3-(AMINOCARBONYL)-1-[(2R,3R,4S,5R)-5-({[(S)-{[(S)-{[(2R,3S,4R,5R)-5-(2-AMINO-6-OXO-1,6-DIHYDRO-9H-PURIN-9-YL)-3,4-DIHYDROXYTETRAHYDROFURAN-2-YL]METHOXY}(HYDROXY)PHOSPHORYL]OXY}(HYDROXY)PHOSPHORYL]OXY}METHYL)-3,4-DIHYDROXYTETRAHYDROFURAN-2-YL]PYRIDINIUM 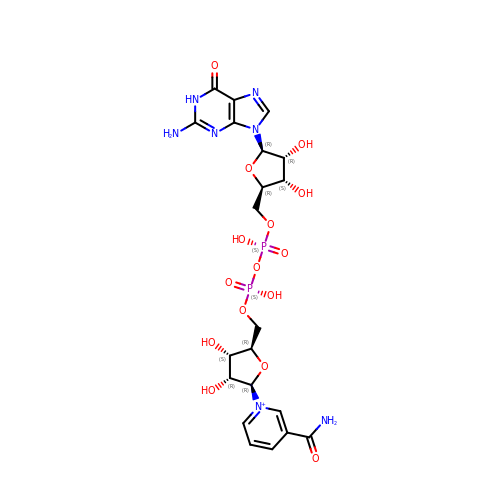| C21 H28 N7 O15 P2 | NCFRZZVNRVEQJK-NAJQWHGHSA-O(S)-cyclopropyl(4-methoxyphenyl)pyrimidin-5-ylmethanol | C15 H16 N2 O2 | 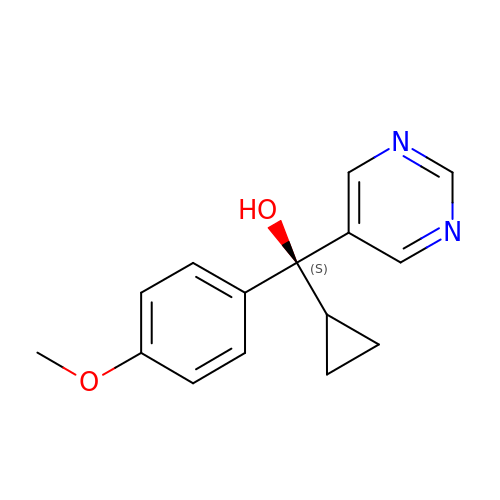HUTDUHSNJYTCAR-HNNXBMFYSA-N>AAADGDDSLYPIAVLIDELRNEDVQLRLNSIKKLSTIALALGVERTRSELLPFLTDTIYDEDEVLLALAEQLGTFTTLVGGPEYVHCLLPPLESLATVEETVVRDKAVESLRAISHEHSPSDLEAHFVPLVKRLAGGDWFTSRTSACGLFSVCYPRVSSAVKAELRQYFRNLCSDDTPMVRRAAASKLGEFAKVLELDNVKSEIIPMFSNLASDEQDSVRLLAVEACVNIAQLLPQEDLEALVMPTLRQAAEDKSWRVRYMVADKFTELQKAVGPEITKTDLVPAFQNLMKDCEAEVRAAASHKVKEFCENLSADCRENVIMSQILPCIKELVSDANQHVKSALASVIMGLSPILGKDNTIEHLLPLFLAQLKDECPEVRLNIISNLDCVNEVIGIRQLSQSLLPAIVELAEDAKWRVRLAIIEYMPLLAGQLGVEFFDEKLNSLCMAWLVDHVYAIREAATSNLKKLVEKFGKEWAHATIIPKVLAMSGDPNYLHRMTTLFCINVLSEVCGQDITTKHMLPTVLRMAGDPVANVRFNVAKSLQKIGPILDNST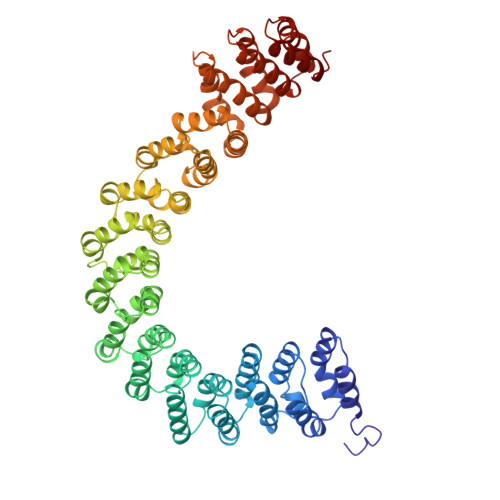LQSEVKPILEKLTQDQDVDVKYFAQEALTVLSLA[2x]> STVEYST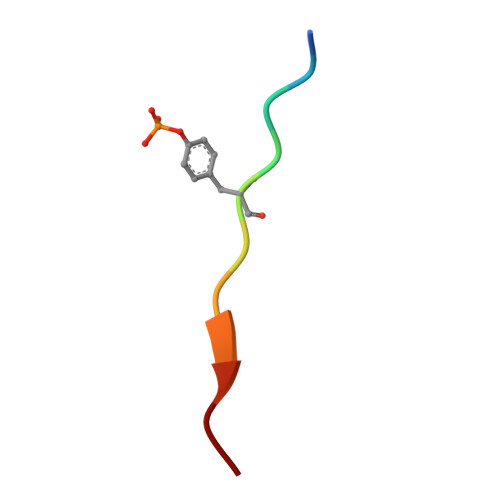VVHS>MAFNGAQTVIQKISWLRTAIAFLKGYMETTGATKKELEQVEKLKERVDEIA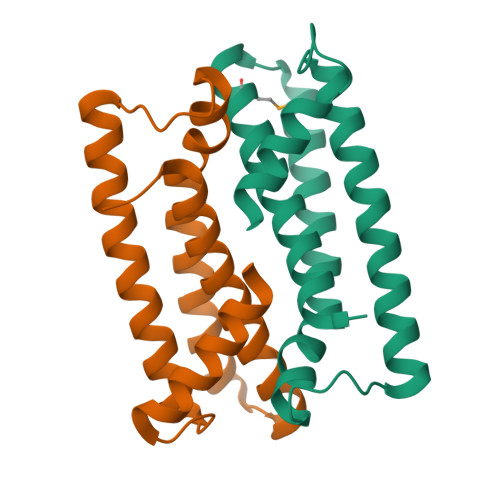TAVNWDVYAQYARGDFNLLSDDEYKEIQKALLVLEDIKEQIIVEMLRVGLAQGQMGTLKISDYLDSLDSHHHHHH[2x]2-methoxy-N-[(3S)-3-methyl-1,1-dioxo-1lambda~6~-thiolan-3-yl]acetamide | C8 H15 N O4 S | 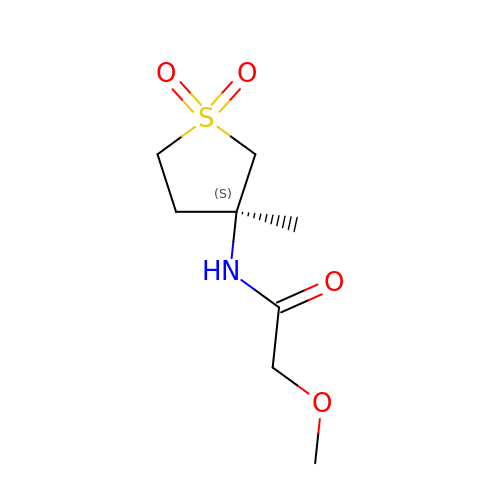INPHJGKASHJNDO-QMMMGPOBSA-N> MKRNYILGLAIGITSVGYGIIDYETRDVIDAGVRLFKEANVENNEGRRSKRGARRLKRRRRHRIQRVKKLLFDYNLLTDHSELSGINPYEARVKGLSQKLSEEEFSAALLHLAKRRGVHNVNEVEEDTGNELSTKEQISRNSKALEEKYVAELQLERLKKDGEVRGSINRFKTSDYVKEAKQLLKVQKAYHQLDQSFIDTYIDLLETRRTYYEGPGEGSPFGWKDIKEWYEMLMGHCTYFPEELRSVKYAYNADLYNALNDLNNLVITRDENEKLEYYEKFQIIENVFKQKKKPTLKQIAKEILVNEEDIKGYRVTSTGKPEFTNLKVYHDIKDITARKEIIENAELLDQIAKILTIYQSSEDIQEELTNLNSELTQEEIEQISNLKGYTGTHNLSLKAINLILDELWHTNDNQIAIFNRLKLVPKKVDLSQQKEIPTTLVDDFILSPVVKRSFIQSIKVINAIIKKYGLPNDIIIELARGGSYATRGLMNLLRSYFRVNNLDVK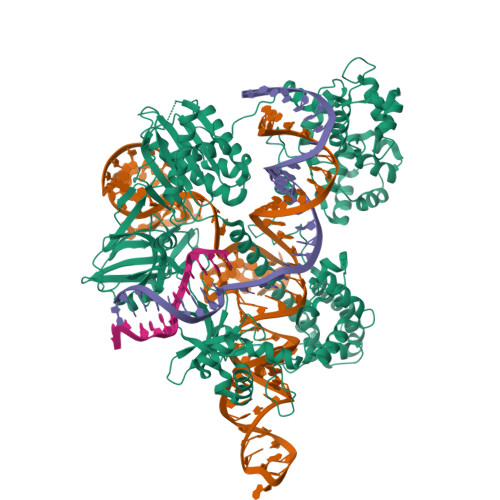VKSINGGFTSFLRRKWKFKKERNKGYKHHAEDALIIANADFIFKEWKKLDKAKKVMENQMFEEKQAESMPEIETEQEYKEIFITPHQIKHIKDFKDYKYSHRVDKKPNRELINDTLYSTRKDDKGNTLIVNNLNGLYDKDNDKLKKLINKSPEKLLMYHHDPQTYQKLKLIMEQYGDEKNPLYKYYEETGNYLTKYSKKDNGPVIKKIKYYGNKLNAHLDITDDYPNSRNKVVKLSLKPYRFDVYLDNGVYKFVTVKNLDVIKKENYYEVNSKCYEEAKKLKKISNQAEFIASFYNNDLIKINGELYRVIGVNNDLLNRIEVNMIDITYREYLENMNDKRPPRIIKTIASKTQSIKKYSTDILGNLYEVKSKKHPQIIKKG> XDN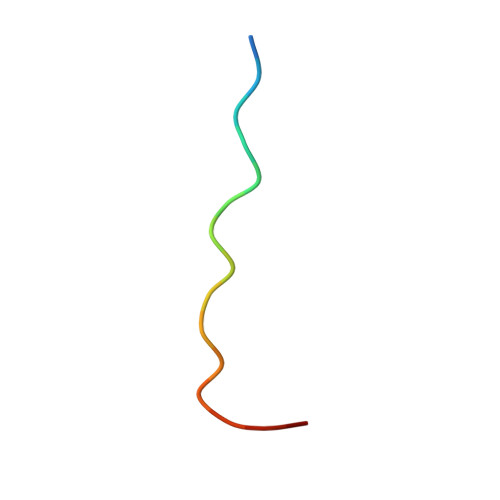SPPPALPKKRQSYX> MALSMTGGQQMGRGSMSRDPLPFFPPLYLGGPEITTENCEREPIHIPGSIQPHGALLTADGHSGEVLQMSLNAATFLGQEPTVLRGQTLAALLPEQWPALQAALPPGCPDALQYRATLDWPAAGHLSLTVHRVGELLILEFEPTEAWDSTGPHALRNAMFALESAPNLRALAEVATQTVRELTGFDRVMLYKFAPDATGEVIAEARREGLHAFLGHRFPAS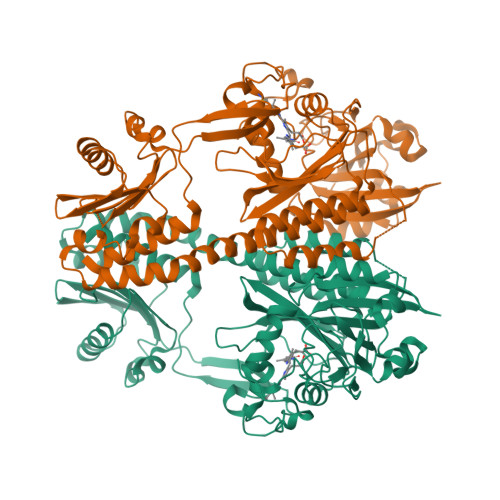DIPAQARALYTRHLLRLTADTRAAAVPLDPVLNPQTNAPTPLGGAVLRATSPMHMQYLRNMGVGSSLSVSVVVGGQLWGLIACHHQTPYVLPPDLRTTLEYLGRLLSLQVQVKEAADVAAFRQSLREHHARVALAAAHSLSPHDTLSDPALDLLGLMRAGGLILRFEGRWQTLGEVPPAPAVDALLAWLETQPGALVQTDALGQLWPAGADLAPSAAGLLAISVGEGWSECLVWLRPELRLEVAWGGATPDQAKDDLGPRHSFDTYLEEKRGYAEPWHPGEIEEAQDLRDTLTGALEHHHHHH>[7x]SDKIIHLTDDSFDTDVLKADGAILVDFWAEWCGPCKMIAPILDEIADEYQGKLTVA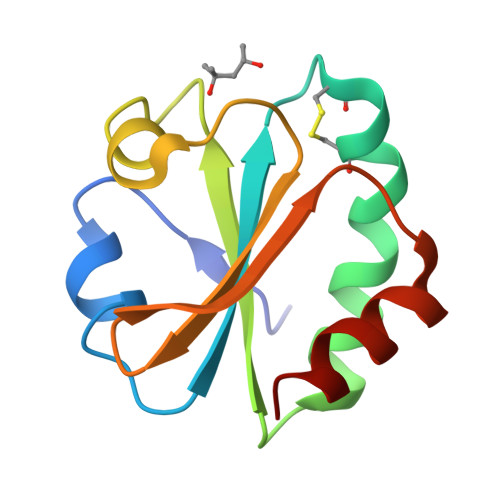KLNIDQNPGTAPKYGIRSIPTLLLFKNGEVAATKVGALSKGQLKEFLDANLA>MSFINYSSREINCKIVYYGPGLCGKTTNLQYIYNKTAAETKGKLISLSTETDRTLFFDFLPLSLGEIRGFKTRFHLYTVPGQVFYDASRKLILKGVDGVVFVADSQIERMEANMESLENLRINLAEQGYDLNKIPYVIQYNKRDLPNAVTVEEMRKALNHRNIPEY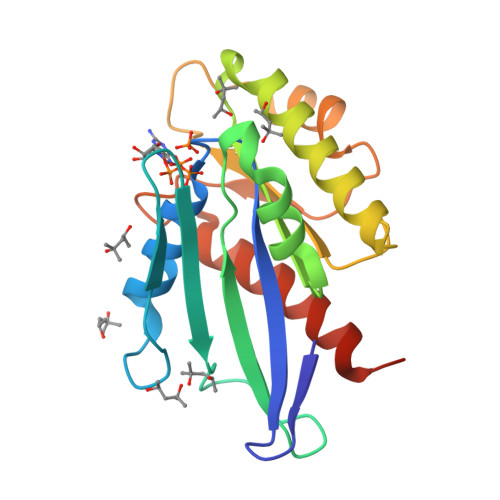QAVAPTGVGVFDTLKAVAKLVLTELKKGGHHHHHH[2x]> MILDTDYITEDGKPVIRIFKKENGEFKIEYDRTFEPYFYALLKDDSAIEEVKKITAERHGTVVTVKRVEKVQKKFLGRPVEVWKLYFTHPQDVPAIRDKIREHPAVIDIYEYDIPFAKRYLIDKGLVPMEGDEELKMLAFAIATLYHEGEEFAEGPILMISYADEEGARVITWKNVDLPYVDVVSTEREMIKRFLRVVKEKDPDVLITYNGDNFDFAYLKKRCEKLGINFALGRDGSEPKIQRMGDRFAVEVKGRIHFDLYPVIRRTINLPTYTLEAVYEAVFGQPKEKVYAEEITTAWETGENLERVARYSMEDAKVTYELGKEFLPMEAQLSRLIGQSLWDVSRSSTGNLVEWFLLRKAYERNELAPNKPDEKELARRRQSYEGGYVKEPERGLWENIVYLDFRSLYPSIIITHNVSPDTLNREGCKEYDVAPQVGHRFCKDFPGFIPSLLGDLLEERQKIKKKMKATIDPIERKLLDYRQRRIKILANSYYGYYGYARARWYCKECAESVTAWGREYITMTIKEIEEKYGFKVIYSDTDGFFATIPGADAETVKKKAMEFLKYINAKLPGALELEYEGFYKRGFFVTKKKYAVIDEEGKITTRGLEIVRRDWSEIAKETQARVLEALLKDGDVEKAVRIVKEVTEKLSKYEVPPEKLVIHIQITRDLKDYKATGPHVAVAKRLAARGVKIRPGTVISYIVLKGSGRIGDRAIPFDEFDPTKHKYDAEYYIENQVLPAVERILRAFGYRKEDLRYQKTRQVGLSAWLKPKGT

Kod-RI is an engineered TNA polymerase that was evolved from a replicative B-family DNA polymerase isolated from the archaeal hyperthermophilic species Thermococcus kodakarensis (Kod). The polymerase harbors the A485R and E664I mutations required for TNA synthesis on DNA templates, as well as the 3′,5′-exonuclease silencing mutations (D141A, E143A) that prevent the removal of newly added TNA residues. Phosphonomethylthreosyl nucleic acid (pTNA, also abbreviated PMT and tPhoNA) is considered a possible XNA candidate for information storage in cellular systems. pTNA is an unusual example of an XNA; it contains modifications in both the sugar and phosphodiester moieties with α-l-threofuranosyl sugars connected by 3′→2′ phosphonomethyl backbone linkages. X-ray crystal structures of the post-catalytic complex showing Kod-RI bound to a DNA substrate that had been extended with either two pTNA adenosine residues (ptA) or two 2′-deoxyadenosine residues (dA) were solved to high resolution.

Our findings indicate that Kod-RI is capable of synthesizing trace amounts of full-length pTNA after 24 h of incubation at 55°C. The nucleotide addition products reside in the enzyme active site of Kod-RI as canonical Watson–Crick base pairs with their complementary thymine bases on the DNA template. Close inspection of the newly added residues failed to identify any differences in the hydrogen bonding pattern of the Watson–Crick base pair even though pTNA does not form a stable duplex with DNA in solution. No signs of duplex destabilization were observed in the pTNA structure, indicating that Kod-RI likely forces pTNA–DNA hybridization by acting as a large molecular clamp to hold the complementary pTNA and DNA strands together. In the Kod-RI structure of the pTNA extended primer, we observe a novel alternative conformation for R606 (labeled R606B) that is not present in the Kod-RI structures solved for the DNA or TNA extended primers. Located on β26 of the thumb subdomain, the positively charged guanidino group of R606B forms a strong ion pair interaction with the negatively charged phosphonate group connecting the newly added ptA12 and ptA13 nucleotides. Other structural differences observed in the polymerase active site include a bridging water interaction between Y594 and the phosphate group linking ptA12 and ptA13 of the pTNA extended structure. Another novel interaction observed in the pTNA extended structure is a weak hydrogen bond between K592 and the O4′ atom on the sugar moiety of ptA13. Additionally, we noticed that the catalytic aspartate D542 was located further away from the terminal pTNA residue than its position in the all-DNA extended structure of Kod-RI, suggesting that the incoming ptNDP substrate may adopt a suboptimal geometry in the enzyme active site. In contrast, the threose ring of pTNA adopts a sugar conformation that is C3′-endo (PptA13 = 37°) and C4′-exo (PptA12 = 47°) in the enzyme active site of Kod-RI.>DPFTMFEEINDFETAFKRLLNEVLEFDLQNPLKDVKKVLCIEPHPDDCVIGMGGTIKRLTDRGIEVIYICMTDGYMGTTDENITGHELAQIRRKEEEESAKMLGVKKIYWLNYRDTELPYSREVRKDLVKIIRKEKPDGVFLPDPWLPYEAHPDHRATGFLALDAV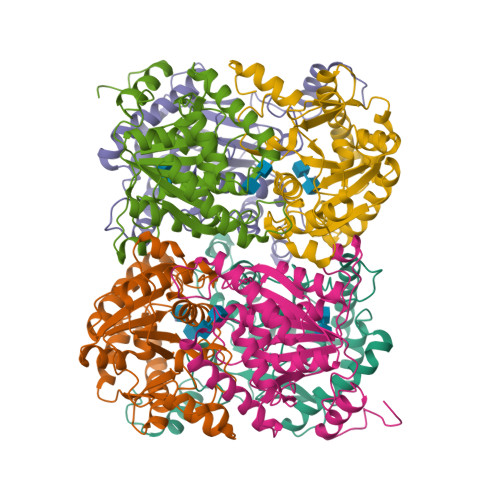AFSPLPNFSNIDLDIGLKPHSVSFIGLYYTSRPNYFVDITDVMDLKLKAIRAHKSQFPDDIWETWEPFLRTVALYYGQKAGVKYAEGFRIMPGLFYHITPFAELI[12x]> TIGPVTPLDASDFALDIRMPGVTPKESDTYFCMSMRLPVDEEAFVIDFKPRASMDTVHHMLLFGCNMPSSTGSYWFCDEG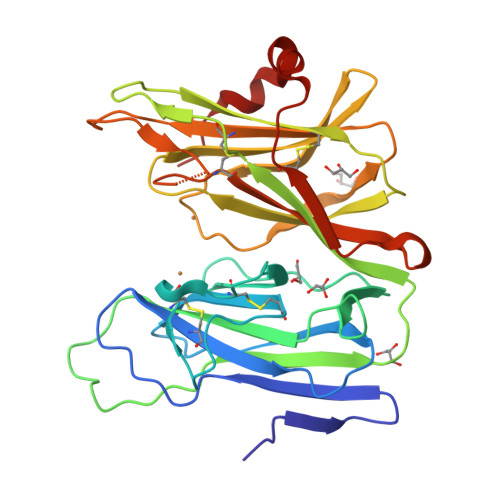TCTDKANILYAWARNAPPTRLPKGVGFRVGGETGSKYFVLQVHYGDISAFRDNHKDCSGVSVHLTRVPQPLIAGMYLMMSVDTVIPPGEKVVNADISCQYKMYPMHVFAYRVHTHHLGKVVSGYRVRNGQWTLIGRQNPQLPQAFYPVEHPVDVTFGDILAARCVFTGEGRTEATHIGGTSSDEMCNLYIMYYMEAKYALSFMTCTKNVAPDMFRTIPAEANIPIP>MSRVSTAPSGKPTAAHALLSRLRDHGVGKVFGVVGREAASILFDEVEGIDFVLTRHEFTAGVAADVLARITGRPQACWATLGPGMTNLSTGIATSV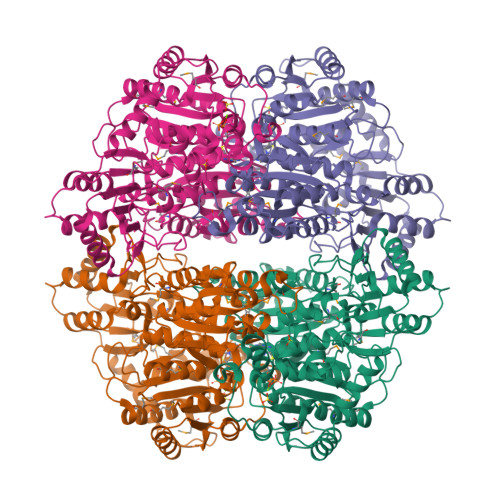LDRSPVIALAAQSESHDIFPNDTHQCLDSVAIVAPMSKYAVELQRPHEITDLVDSAVNAAMTEPVGPSFISLPVDLLGSSEGIDTTVPNPPANTPAKPVGVVADGWQKAADQAAALLAEAKHPVLVVGAAAIRSGAVPAIRALAERLNIPVITTYIAKGVLPVGHELNYGAVTGYMDGILNFPALQTMFAPVDLVLTVGYDYAEDLRPSMWQKGIEKKTVRISPTVNPIPRVYRPDVDVVTDVLAFVEHFETATASFGAKQRHDIEPLRARIAEFLADPETYEDGMRVHQVIDSMNTVMEEAAEPGEGTIVSDIGFFRHYGVLFARADQPFGFLTSAGCSSFGYGIPAAIGAQMARPDQPTFLIAGDGGFHSNSSDLETIARLNLPIVTVVVNNDTNGLIELYQNIGHHRSHDPAVKFGGVDFVALAEANGVDATRATNREELLAALRKGAELGRPFLIEVPVNYDFQPGGFGALSI[4x]> MKTQVAIIGAGPSGLLLGQLLHKAGIDNVILERQTPDYVLGRIRAGVLEQGMVDLLREAGVDRRMARDGLVHEGVEIAFAGQRRRIDLKRLSGGKTVTVYGQTEVTRDLMEAREASGATTVYQAAEVRLHDLQGERPYVTFERDGERLRLDCDYIAGCDGFHGISRQSIPAERLKVFERVYPFGWLGLLADTPPVSHELIYANHPRGFALCSQRSATRSRYAVQVPLTEKVEDWSDERFWTELKARLPAEVAEKLVTGPSLEKSIAPLRSFVVEPMQHGRLFLAGDAAHIVPPTGAKGLNLAASDVSTLYRLLLKAYREGRGELLERYSAICLRRIWKAER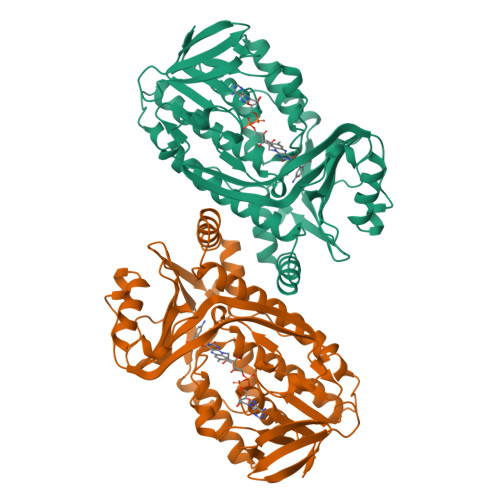FSWWMTSVLHRFPDTDAFSQRIQQTELEYYLGSEAGLATIAENYVGLPYEEIE>[2x]SNGNPDSPRCSKHNRLCILRVVGKDGEN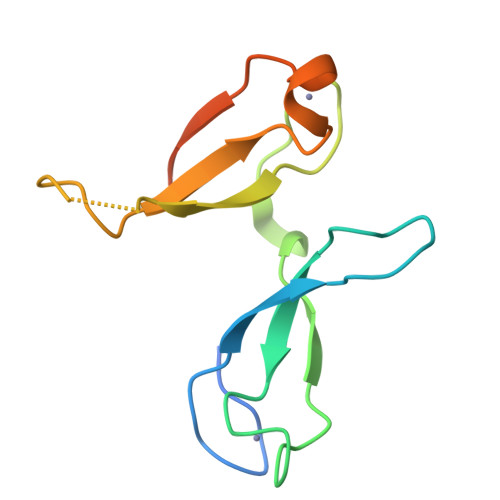KGRQFYACPLPREAQCGFFEWADLSFPFCNHGKRSTMKTVLKIGPNNGKNFFVCPLGKEKQCNFFQWAENGPGIKIIPGC> MALFGSNDVTTAHSDYEIVLEGGSSSWGKVKARAKVNAPPASPLLPADCDVKLNVKPLDPAKGFVRISAVFESIVDSTKNKLTIEADIANETKERRISVGEGMVSVGDFSHTFSFEGSVVNLFYYRSDAVRRNVPNPIYMQGRQFHDILMKVPLDNNDLIDTWEGTVKAIGSTGAFNDWIRDFWFIGPAFTALNEGGQRISRIEVNGLNTESGPKGPVGVSRWRFSHGGSGMVDSISRWAELFPSDKLNRPAQVEAGFRSDSQGIEVKVDGEFPGVSVDAGGGLRRILNHPLIPLVHHGMVGKFNNFNVDAQLKVVLPKGYKIRYAAPQYRSQNLE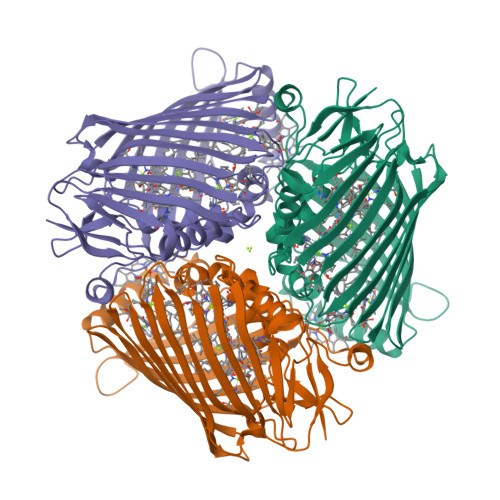EYRWSGGAYARWVEHVCKGGVGQFEILYAQ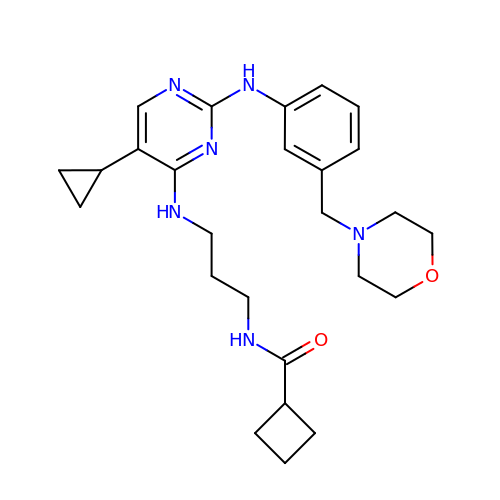N-{3-[(5-cyclopropyl-2-{[3-(morpholin-4-ylmethyl)phenyl]amino}pyrimidin-4-yl)amino]propyl}cyclobutanecarboxamide | C26 H36 N6 O2 | UKBGBACORPRCGG-UHFFFAOYSA-N> MGKGHHHHHHGSERTGTQPLGVQGLTEEQRMMIRELMDAQMKTFDTTFSHFKNFRLPGVLSSGCELPESLQAPSREEAAKWSQVRKDLCSLKVSLQLRGEDGSVWNYKPPADSGGKEIFSLLPHMADMSTYMFKGIISFAKVISYFRDLPIEDQISLLKGAAFELCQLRFNTVFNAETGTWECGRLSYCLEDTAGGFQQLLLEPMLKFHYMLKKLQLHEEEYVLMQAISLFSPDRPGVLQHRVVDQLQEQFAITLKS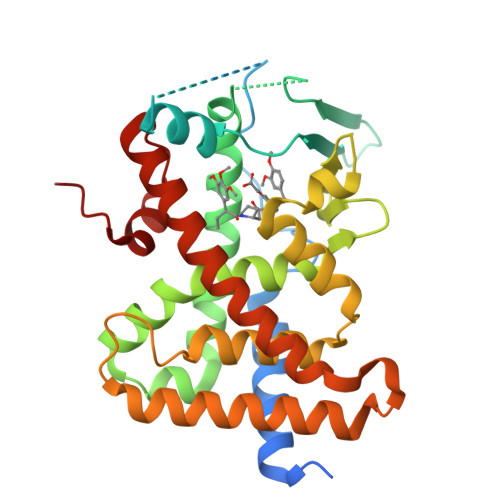YIECNRPQPAHRFLFLKIMAMLTELRSINAQHTQRLLRIQDIHPFATPLMQELFGITGS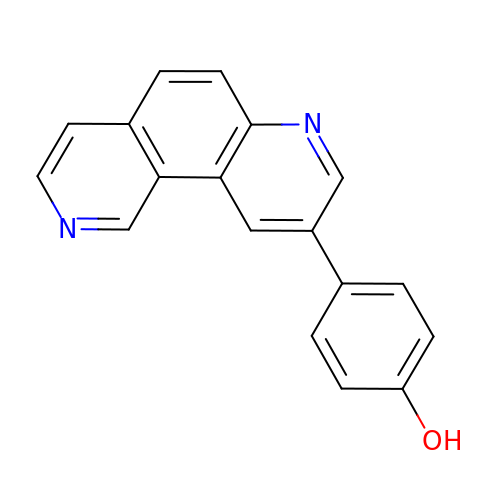9-(4-HYDROXYPHENYL)-2,7-PHENANTHROLINE | C18 H12 N2 O | IUSSGTWHFMSCOY-UHFFFAOYSA-N> MSLKTYKGYLIDLDGTMYNGTEKIEEACEFVRTLKDRGVPYLFVTNNSSRTPKQVADKLVSFDIPATEEQVFTTSMATAQHIAQQKKDASVYVIGEEGIRQAIEENGLTFG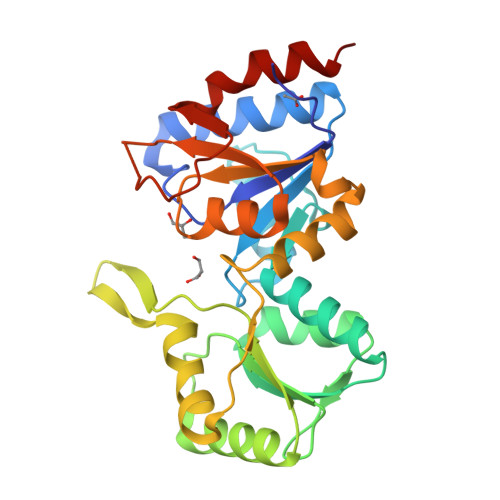GENADFVVVGIDRSITYEKFAVGCLAIRNGARFISTNGDIAIPTERGLLPGNGSLTSVLTVSTGVQPVFIGKPESIIMEQAMRVLGTDVSETLMVGDNYATDIMAGINAGMDTLLVHTGVTKREHMTDDMEKPTHAIDSLTEWIPYIEGHHHHHH> GTSSMGYLMALFEDIQAVIAEQLNVDAAQVTPEAEFV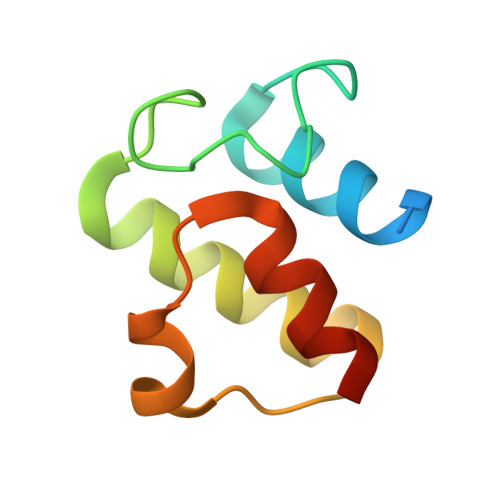KDLGADSLDVVELIMALEEKFGIEIPDEQAEKIVNVGDVVKYIEDNKLA> MGRLLALVVGAALVSSACGGCVEVDSETEAVYGMTFKILCISCKRRSETNAETFTEWTFRQKGTEEFVKILRYENEVLQLEEDERFEGRVVWNGSRGTKDLQDLSIFITNVTYNHSGDYECHVYRLLFFENYEHNTSVVKKIHIEVVDKANRDMASIVSEIMMYVLIVVLTIWLVAEMIYCYKKIAAATETAAQENASEYLAITSESKENCTGVQVAE;> MHRDAWLPRPAFSLTGLSLFFSLVPPGRSMEVTVPATLNVLNGSDARLPCTFNSCYTVNHKQFSLNWTYQECNNCSEEMFLQFRMKIINLKLERFQDRVEFSGNPSKYDVSVMLRNVQPEDEGIYNCYIMNPPDRHRGHGKIHLQVLMEEPPERDSTVAVIVGASVGGFLAVVILVLMVVKCVRRKKEQKLSTDDLKTEEEGKTDGEGNPDDGAK;> MAQALLVPPGPESFRLFTRESLAAIEKRAAEEKAKKPKKEQDNDDENKPKPNSDLEAGKNLPFIYGDIPPEMVSEPLEDLDPYYINKKTFIVMNKGKAIFRFSATSALYILTPLNPVRKIAIKILVHSLFSMLIMCTILTNCVFMTLSNPPDWTKNVEYTFTGIYTFESLIKILARGFCLEDFTFLRDPWNWLDFSVIVMAYVTEFVSLGNVSALRTFRVLRALKTISVIPGLKTIVGALIQSVKKLSDVMILTVFCLSVFALIGLQLFMGNLRNKCLQWPPSDSAFETNTTSYFNGTMDSNGTFVNVTMSTFNWKDYIGDDSHFYVLDGQKDPLLCGNGSDAGQCPEGYICVKAGRNPNYGYTSFDTFSWAFLSLFRLMTQDYWENLYQLTLRAAGKTYMIFFVLVIFLGSFYLVNLILAVVAMAYEEQNQATLEEAEQKEAEFQQMLEQLKKQQEEAQAVAAASAASRDFSGIGGLGELLESSSEASKLSSKSAKEWRNRRKKRRQREHLEGNNKGERDSFPKSESEDSVKRSSFLFSMDGNRLTSDKKFCSPHQSLLSIRGSLFSPRRNSKTSIFSFRGRAKDVGSENDFADDEHSTFEDSESRRDSLFVPHRHGERRNSNVSQASMSSRMVPGLPANGKMHSTVDCNGVVSLVGGPSALTSPTGQLPPEGTTTETEVRKRRLSSYQISMEMLEDSSGRQRAVSIASILTNTMEELEESRQKCPPCWYRFANVFLIWDCCDAWLKVKHLVNLIVMDPFVDLAITICIVLNTLFMAMEHYPMTEQFSSVLTVGNLVFTGIFTAEMVLKIIAMDPYYYFQEGWNIFDGIIVSLSLMELGLSNVEGLSVLRSFRLLRVFKLAKSWPTLNMLIKIIGNSVGALGNLTLVLAIIVFIFAVVGMQLFGKSYKECVCKINDDCTLPRWHMNDFFHSFLIVFRVLCGEWIETMWDCMEVAGQTMCLIVFMLVMVIGNLVVLNLFLALLLSSFSSDNLAATDDDNEMNNLQIAVGRMQKGIDYVKNKMRECFQKAFFRKPKVIEIHEGNKIDSCMSNNTGIEISKELNYLRDGNGTTSGVGTGSSVEKYVIDENDYMSFINNPSLTVTVPIAVGESDFENLNTEEFSSESELEESKEKLNATSSSEGSTVDVVLPREGEQAETEPEEDLKPEACFTEGCIKKFPFCQVSTEEGKGKIWWNLRKTCYSIVEHNWFETFIVFMILLSSGALAFEDIYIEQRKTIKTMLEYADKVFTYIFILEMLLKWVAYGFQTYFTNAWCWLDFLIVDVSLVSLVANALGYSELGAIKSLRTLRALRPLRALSRFEGMRVVVNALVGAIPSIMNVLLVCLIFWLIFSIMGVNLFAGKFYHCVNMTTGNMFDISDVNNLSDCQALGKQARWKNVKVNFDNVGAGYLALLQVATFKGWMDIMYAAVDSRDVKLQPVYEENLYMYLYFVIFIIFGSFFTLNLFIGVIIDNFNQQKKKFGGQDIFMTEEQKKYYNAMKKLGSKKPQKPIPRPANKFQGMVFDFVTRQVFDISIMILICLNMVTMMVETDDQGKYMTLVLSRINLVFIVLFTGEFVLKLVSLRHYYFTIGWNIFDFVVVILSIVGMFLAEMIEKYFVSPTLFRVIRLARIGRILRLIKGAKGIRTLLFALMMSLPALFNIGLLLFLVMFIYAIFGMSNFAYVKKEAGIDDMFNFETFGNSMICLFQITTSAGWDGLLAPILNSAPPDCDPDTIHPGSSVKGDCGNPSVGIFFFVSYIIISFLVVVNMYIAVILENFSVATEESAEPLSEDDFEMFYEVWEKFDPDATQFIEFSKLSDFAAALDPPLLIAKPNKVQLIAMDLPMVSGDRIHCLDILFAFTKRVLGESGEMDALRIQMEDRFMASNPSKVSYEPITTTLKRKQEEVSAAIIQRNFRCYLLKQRLKNISSNYNKEAIKGRIDLPIKQDMIIDKLNGNSTPEKTDGSSSTTSPPSYDSVTKPDKEKFEKDKPEKESKGKEVRENQK

Voltage-gated sodium (NaV) channels generate rapid sodium influx to initiate and propagate action potentials in excitable cells. NaV1.3 is involved in numerous physiological processes including neuronal development, hormone secretion and pain perception. NaVs are composed of a large pore-forming α-subunit and regulatory β-subunits. Here we report structures of human NaV1.3/β1/β2 in complex with clinically-used drug bulleyaconitine A and selective antagonist ICA121431.

To investigate the selectivity and inhibition mechanism of ICA, we determined the cryo-EM structure of NaV1.3/β1/β2-ICA at 3.4-Å resolution. Notably, a strong piece of density was found inside the extracellular aqueous cleft of VSDIV, which is absent in the map of NaV1.3/β1/β2-BLA and agrees well with the ICA molecule. The small sidechains of G1603 on S3 helix (G1603S3) and A1626S4 create room to accommodate the thiazole headgroup. The anionic thiazole directly interacts with three of six gating charges (i.e., R2−R4) through electrostatic interactions. The middle benzene ring contacts L1563S2 and M1604S3 via van der Waals interactions. The protruding diphenyl tail of ICA outside of the binding cleft is further stabilized by R1560S2 and F1605S3. Interestingly, a possible lipid molecule helps to stabilize the hydrophobic tail at a distance of ~4 Å, suggesting that lipid may be involved in this drug-channel interaction. Our structure of the NaV1.3-ICA complex illustrates that, despite high overall structure similarity, S1559 and R1560 are the key determinants for the selective inhibition of ICA on NaV1.3/NaV1.1, which is supported by significant potency reduction of ICA on the S1559Y and R1560W mutants by 9-fold and 33-fold, respectively. Most of the key residues around the receptor site assume nearly identical conformations, R4 of NaV1.3-ICA was slightly pulled upward by the anionic thiazole group. This observation suggests that the ICA binding stabilizes VSDIV in the activated conformation. As a result, the IFM-motif binds to its receptor site, and the activation gate becomes non-conductive for hydrated Na+.>[4x]MKQVCVLGNGQLGRMLRQAGEPLGIAVWPVGLDAEPAAVPFQQSVITAEIERWPETALTRELARHPAFVNRDVFPIIADRLTQKQLFDKLHLPTAPWQLLAERSEWPAVFDRLGELAIVKRRTGGYDGRGQWRLRANETEQLPAECYGECIVEQGINFSGEVSLVGARGFDGSTVFYPLTHNLHQD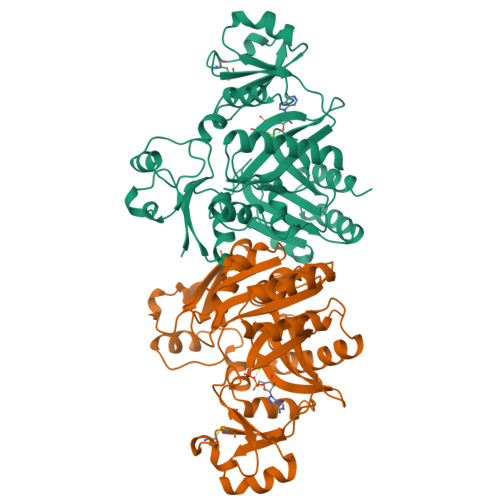GILRTSVAFPQANAQQQARAEEMLSAIMQELGYVGVMAMECFVTPQGLLINELAPRVHNSGHWTQNGASISQFELHLRAITDLPLPQPVVNNPSVMINLIGSDVNYDWLKLPLVHLHWYDKEVRPGRKVGHLNLTDSDTSRLTATLEALIPLLPPEYASGVIWAQSKFG> MDLLKRHLAPIVPDAWSAIDEEAKEIFQGHLAGRKLVDFRGPFGWEYAAVNTGELRPIDDTPEDVDMKLRQVQPLAEVRVPFTLDVTELDSVARGATNPDLDDVARAAERMVEAEDSAIFHGWAQAGIKGIVDSTPHEALAVASVSDFPRAVLSAADTLRKAGVTGPYALVLGPKAYDDLFAATQDG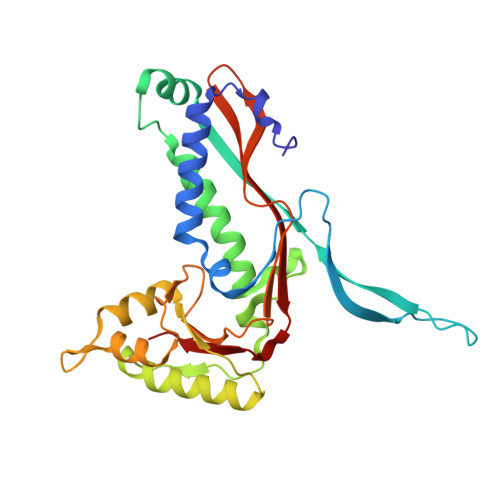YPVAKQVQRLVVDGPLVRANALAGALVMSMRGGDYELTVGQDLSIGYAFHDRSKVELFVAESFTFRVLEPGAAVHLRYA> SPSAQELKEQGNRLFVGRKYPEAAACYGRAITRNPLVAVYYTNRALCYLKMQQHEQALADCRRALEL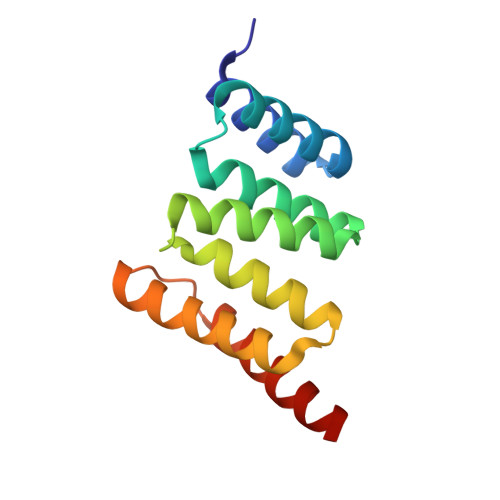DGQSVKAHFFLGQCQLEMESYDEAIANLQRAYSLAKEQRLNFGDDIPSALRIAKKKRWNSIEE> SSQIRQNYSTEVEAAVNRLVNLYLRASYTYLSLGFYFDRDDVALEGVCHFFCELACEKCEGACRLLKMQNQRGGRALFQDLQKPSQDEWGTTLDAMKAAIVLEKSLNQALLDLHALGSAQADPHLCDFLESHFLDEEVK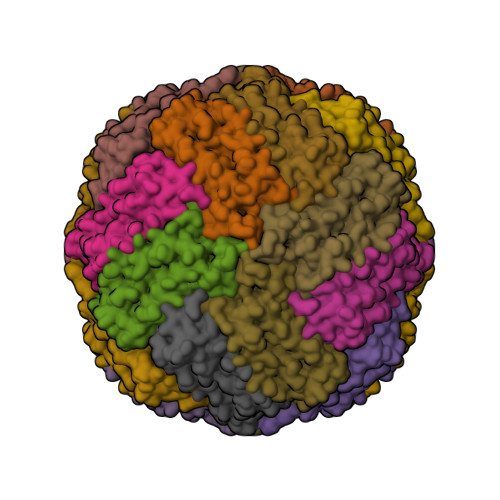LIKKMGDHLTNIQRLVGSQAGLGEYLFERLTLKHD>[2x]HHHHHHFNLPPGNYKKPKLLYCSNGGHFLRILPDGTVDGTRDRSDQHIQLQLSA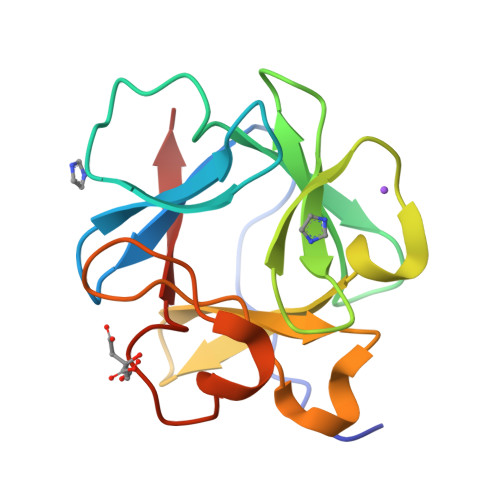ESVGEVYIKSTETGQYLAMDTDGLLYGSQTPNEECLFLERLEENHYNTYISKKHAEKNWFVGLKKNGSSKRGPRTHYGQKAILFLPLPVSSD> GSHMQSYQISSRLMAQEGQRTSVQTSSLIQSLFDFRLAALRIHQDSTAKNASLINALVSRDSSRLDEFFSSVDELELSNAPDLRFISSHDNILWDDGNASFYGIAQQE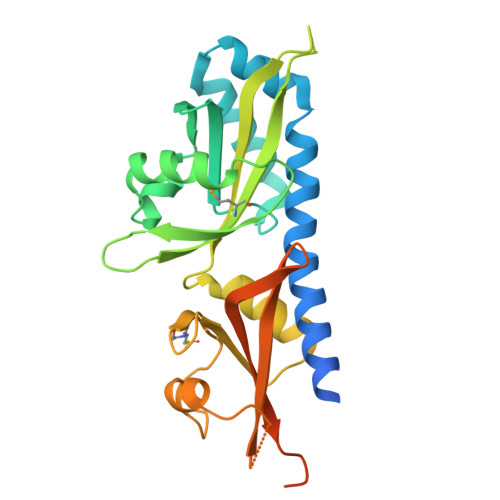LNKLIRRVAISGNWHLVQTPSEGKSVHILMRRSSLIEAGTGQVVGYLYVGIVLNDNFALLENIRSGSNSENLVLAVDTTPLVSTLKGNEPYSLDYVVHSAKDAMRDSFIVGQTFLEVESVPTYLCVYSIQTNQNVLTLRDNESVPTYLCVYSIQTNQNVRHQ Ginsenoside Rh2 | C36 H62 O8 | 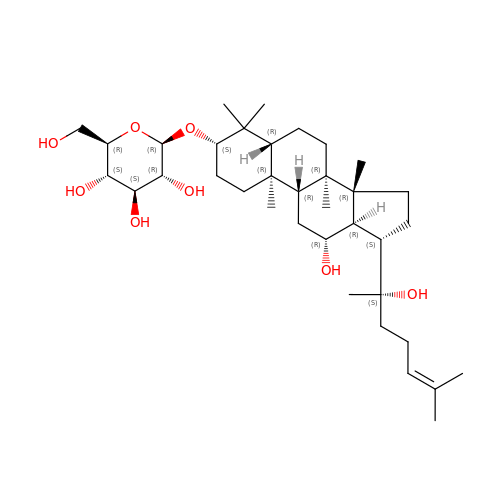CKUVNOCSBYYHIS-IRFFNABBSA-N>[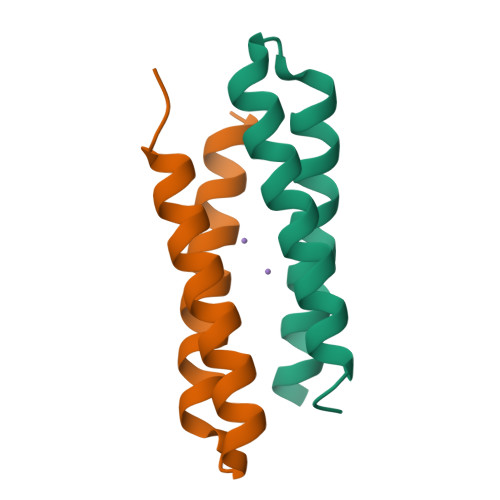2x]DYLRELYKLEQQAMKLYREASEKARNPEKKSVLQKILEDEEKHIEWLETIN>GSPEFIEKNFVITDPRLPDNPIIFASDGFLELTEYSREEILGRNARFLQGPETDQATVQKIRDAIRDQRETTVQLINYTKSGKKFWNLLHLQPVRDQKGELQYFIGVQLDGS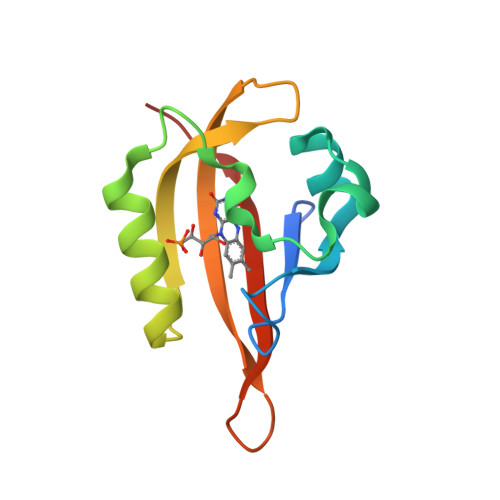DHV[2x]>GMDTSPTKAVSSAPTIVDVDLGDRSYPIYIGSGLLDQPDLLQRHVHGKRVLVVTNSTVAPIYLDKVVGALTNENPNVSVESVILPDGEKYKNMDTLMKVFDKAIESRLDRRCTFVALGGGVIGDMCGYAAASFLRGVNFIQIPTTVMAQVDSSVGGKTGINHRLGKNLIGAFYQPQCVLIDTDTLNTLPDRELASGLAEVVKYGLIRDANFFEWQEKNMPALMARDPSALAYAIKRSCENKAEVVSLDEKESGLRATLNLGHTFGHAIETGFGYGQWLHGEAVAAGMVMAVDMSYRLGWID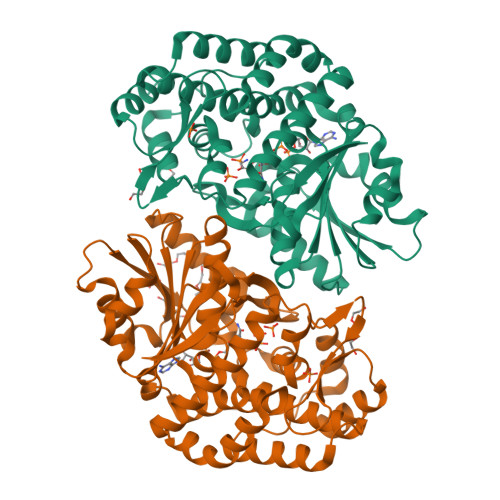ESIVNRAHNILQQAKLPTAPPETMTVEMFKSVMAVDKKVADGLLRLILLKGPLGNCVFTGDYDRKALDETLHAFCKS[4x]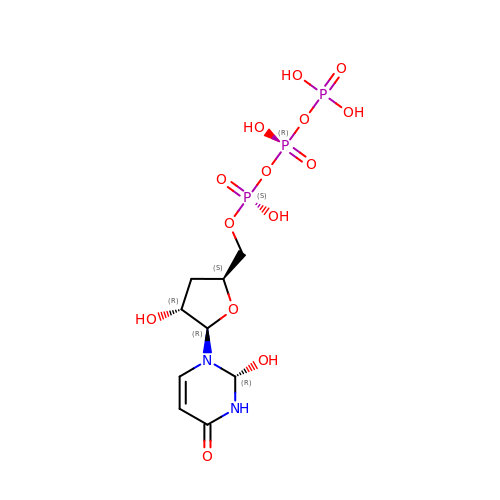3'-DEOXY-URIDINE 5'-TRIPHOSPHATE | C9 H17 N2 O14 P3 | CVEDUOUYNXHQBA-HIORRCEOSA-N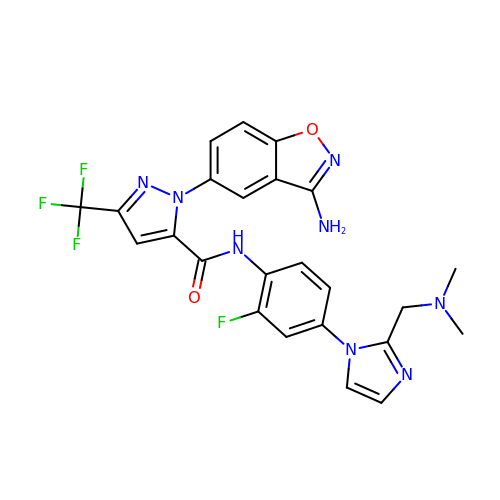1-(3-AMINO-1,2-BENZISOXAZOL-5-YL)-N-(4-{2-[(DIMETHYLAMINO)METHYL]-1H-IMIDAZOL-1-YL}-2-FLUOROPHENYL)-3-(TRIFLUOROMETHYL)-1H-PYRAZOLE-5-CARBOXAMIDE | C24 H20 F4 N8 O2 | OFJRNBWSFXEHSA-UHFFFAOYSA-N> GAMDPEFLDPNLPPSSNFDLSAWYLSVPTDNNGDGKADSIKENDLNAGYADGTYFYTAADGGMVFRCPIDGYKTSTNTSYTRTELREMLRRGDTSIATQGVNGNNWVFGSAPASAREAAGGVDGVLRATLAVNHVTTTGDSG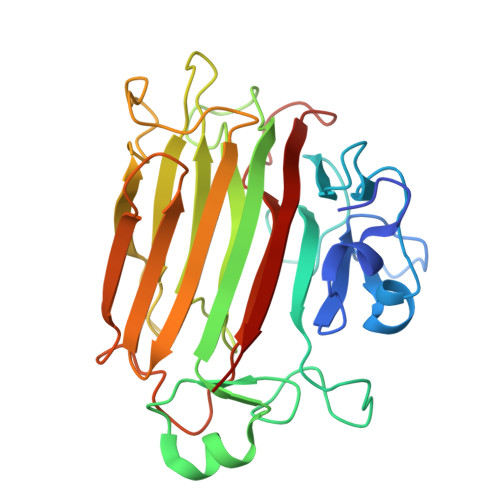QVGRVIVGQIHANNDEPLRLYYRKLPGHSKGSVYIAHEPNGGSDSWYDMIGSRSSSASDPSDGIALDEVWSYEVKVVGNTLTVTIFRAGKDDVVQVVDMGNSGYDVADQYQYFKAGVYNQNNTGNASDYVQVTFYALEQSHD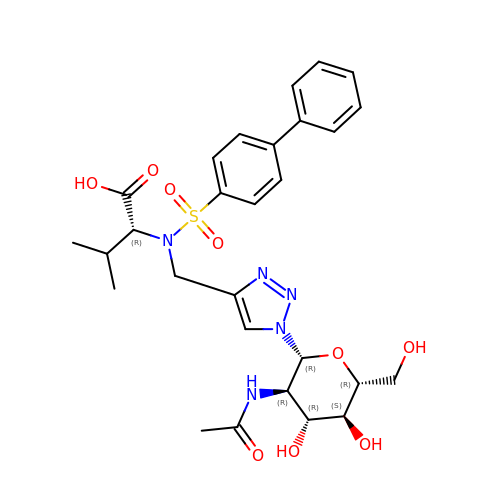N-({1-[2-(acetylamino)-2-deoxy-beta-D-glucopyranosyl]-1H-1,2,3-triazol-4-yl}methyl)-N-[([1,1'-biphenyl]-4-yl)sulfonyl]-D-valine | C28 H35 N5 O9 S | KNBZJXWGCBPDHT-ZRRJEQDASA-N(2~{S},3~{R},4~{S},5~{R})-5-(hydroxymethyl)-3,4-bis(oxidanyl)-~{N}-pentyl-pyrrolidine-2-carboxamide | C11 H22 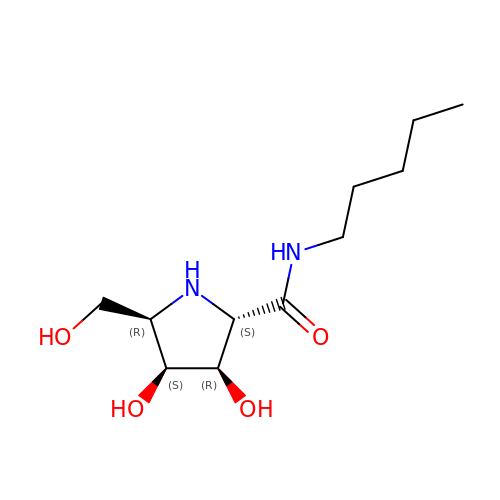N2 O4 | QKDMGVVHKYSWEM-XFWSIPNHSA-N> GSMGSKRQWALEDFEIGRPLGKGKFGNVYLAREKQSKFILALKVLFKAQLEKAGVEHQLRREVEIQSHLRHPNILRLYGYFHDATRVYLILEYAPLGTVYRELQKLSKFDEQRTATYITELANALSYCHSKRVIHRDIKPENLLLGSAGELKIADFGWSVHAPSSRRTTLCGTLDYLPPEMIEGRMHDEKVDLWSLGVLCYEFLVGKPPFEANTYQETYKRISRVEFTFPDFVTEGARDLISRLLKHNPSQRPMLREVLEHPWITANSSKPS

Aurora A is one of three human aurora kinases, a family of serine/threonine kinases that play a central role in cell division. During mitosis, Aurora A is localized to microtubules in the mitotic spindle through an interaction between the kinase domain and the protein TPX2.15 The N-terminal sequence of TPX2 binds to an allosteric pocket on Aurora A16 and stimulates kinase activity, leading to cell-cycle progression. Interruption of the Aurora A–TPX2 interaction reduces kinase activity, leading to mislocalization of Aurora A, mitotic defects, and cell cycle arrest. In previous work, some of us have described the development of small-molecule inhibitors targeting the TPX2 binding pocket of Aurora A.18 In particular, through a process of high-throughput screening of diverse chemical libraries and fragment deconstruction, the fragment 2-phenyl-4-carboxyquinoline (compound 1) was developed.

A process of synthesis and investigation of structure–activity relationship (SAR) trends was embarked upon to improve the potency of the fragment, mainly through increasing the hydrophobicity of the phenyl group which occupies the pocket formed by residues L178, V182, V206 and L208. In general, it can be seen that adding halogens at the position X is predicted to be favorable. In order to check the orientation of the small molecules in the binding pocket, we have collected X-ray crystal structures of 2 and 5 (see the ESI†). In contrast to the MC simulations, both crystal structures clearly show that φ is close to 180°. The discrepancy is possibly due to force field inaccuracy, crystallization conditions, or a small population of alternative conformations may not be visible in the X-ray electron density. It is more difficult to assign the orientation of the L178 side chain, and so the inter-conversion between the two populations observed in the MC simulations may be accurate. As predicted, compound 9 also shows enhanced activity relative to 2.Middle East respiratory syndrome coronavirus (MERS-CoV) and the pangolin MERS-like coronavirus MjHKU4r-CoV-1 employ dipeptidyl peptidase 4 (DPP4) as an entry receptor. To understand the mechanism of MjHKU4r-CoV-1 entry into cells, we determined the crystal structures of the receptor binding domain (RBD) of MjHKU4r-CoV-1 spike protein bound to human DPP4 (hDPP4) and Malayan pangolin DPP4 (MjDPP4), respectively. MjHKU4r-CoV-1 RBD is composed of a core structure and an external domain. The structure of hDPP4 or MjDPP4 consists of a α/β hydrolase domain and an eight-bladed β propeller domain. Both DPP4 receptors bind to MjHKU4r-CoV-1 RBM via blades IV and V of their β propeller domains, in agreement with the complex structures of MERS-CoV RBD-hDPP4 and Ty-BatCoV-HKU4 RBD-hDPP4 solved previously.

The crystals of the MjHKU4r-RBD and hDPP4 complex were obtained in 0.1 M HEPES (pH 7.0) and 10% (wt/vol) PEG 6000. The two MjHKU4r-CoV-1 RBD-hDPP4 heterocomplexes in the ASU are also similar to each other (RMSD of 0.787 Å over 944 aligned Cα atoms). The overall hDPP4-binding mode of MjHKU4r-CoV-1 RBD is similar to that of MERS-CoV RBD. As expected, the footprint of MjHKU4r-CoV-1 RBD on hDPP4 largely overlaps with those of MERS-CoV RBD and Ty-BatCoV-HKU4 RBD. As MjHKU4r-CoV-1 RBD is orientated differently on hDPP4 and MjDPP4, there are also interactions specific to each complex. The RBD residue D471 only forms a salt bridge interaction with hDPP4 R336. In the MjHKU4r-CoV-1 RBD-hDPP4 complex, D545 forms ionic interactions with K267 of hDPP4 and therefore D545 plays a similar role as E544 in the MjHKU4r-CoV-1 RBD-MjDPP4 complex. For instance, D471 on MjHKU4r-CoV-1 RBD forms a strong salt bridge interaction with R336 of hDPP4. H517N mutation on MjHKU4r-CoV-1 RBD significantly reduced protein binding and MjHKU4r-CoV-1 pseudovirus infection, as this mutation would likely break the hydrogen bonding between the side chain of H517 and the NAG linked to N321 of hDPP4. The SPR assay showed that the affinity of MjHKU4r-CoV-1 RBD to hDPP4 was about 20-fold higher than that of Ty-BatCoV-HKU4 RBD to hDPP4, implying the former virus was probably more adapted to human DPP4 receptor.

>[2x]DSRKTYTLTDYLKNTYRLKLYSLRWISDHEYLYKQENNILVFNAEYGNSSVFLENSTFDEFGHSINDYSISPDGQFILLEYNYVKQWRHSYTASYDIYDLNKRQLITEERIPNNTQWVTWSPVGHKLAYVWNNDIYVKIEPNLPSYRITWTGKEDIIYNGITDWVYEEEVFSAYSALWWSPNGTFLAYAQFNDTEVPLIEYSFYSDESLQYPKTVRVPYPKAGAVNPTVKFFVVNTDSLSSVTNATSIQITAPASMLIGDHYLCDVTWATQERISLQWLRRIQNYSVMDICDYDESSGRWNCLVARQHIEMSTTGWVGRFRPSEPHFTLDGNSFYKIISNEEGYRHICYFQIDKKDCTFITKGTWEVIGIEALTSDYLYYISNEYKGMPGGRNLYKIQLSDYTKVTCLSCELNPERCQYYSVSFSKEAKYYQLRCSGPGLPLYTLHSSVNDKGLRVLEDNSALDKMLQNVQMPSKKLDFIILNETKFWYQMILPPHFDKSKKYPLLLDVYAGPCSQKADTVFRLNWATYLASTENIIVASFDGRGSGYQGDKIMHAINRRLGTFEVEDQIEAARQFSKMGFVDNKRIAIWGWSYGGYVTSMVLGSGSGVFKCGIAVAPVSRWEYYDSVYTERYMGLPTPEDNLDHYRNSTVMSRAENFKQVEYLLIHGTADDNVHFQQSAQISKALVDVGVDFQAMWYTDEDHGIASSTAHQHIYTHMSHFIKQCFSLP;>[2x]KECDFTPMLVGVPPQVYNFKRLVFTNCNYNLTKLLSLFMVNEFSCNGISPDAIARGCYSSLTVDYFAYPLSMRSYIQPGSAGDISLYNYKQSFANPTCRVLATAPANLTLTKPSAYGYFQKCSRVSGEHNSVETPLYINPGEYSICRSFSPYGFSEDGEVFRRQLTQYEGGGILVGVGAKLAMTDKLEMGFIISVQYGTDTNSVCPML>[4x]MQTALTTRDSFDPFASTRTFNLAMTDIGEMYFMPPLMEALAQRAPHIQISTLRPNAGNLKE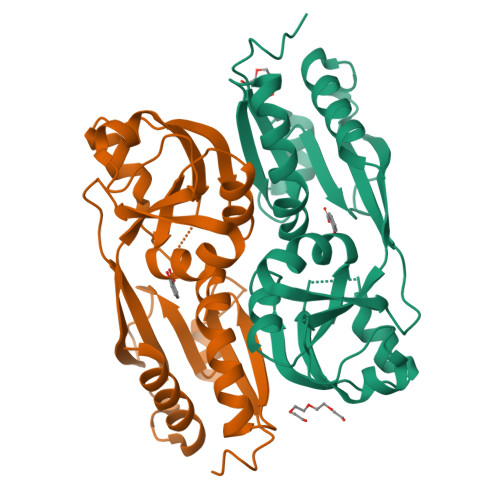DMESGAVDLALGLLPELQTGFFQRRLFRHRYVCMFRKDHPSAKSPMSLKQFTELEHVGVVALNTGHGEVDGLLERAGIKRRMRLVVPHFIAIGPILHSTDLIATVPQRFAVRCEVPFGLTTSPHPAKLPDIAINLFWHAKYNRDPGNMWLRQLFVELFSEAHHHHHH>[12x]SVDTMALWLGLRAVLVVAGLAVLLQLIRGWLSSKSYVFNREEIARLAKEHSGLDYEVAFSKI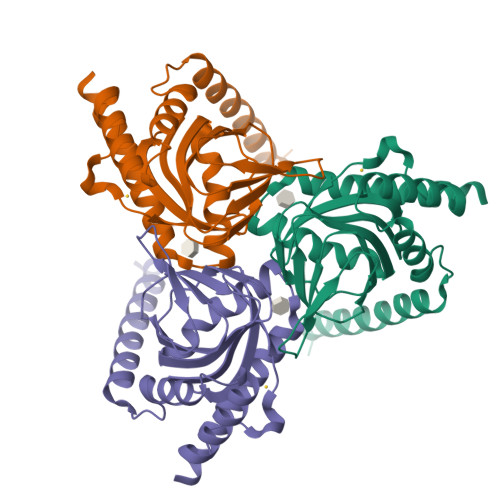IVELRKKHPGHILQDEDLQWVFVNAGGWMGSMCLLHASLTEYVLLFGTAVDTGGHSGRYWAEISDTILSGTFRQWKEGTTKSEIFYPGDTIVHEVGEATSVQWSSGTWMVEYGRGFIPSTLAFALADTIFSTQDFLTLFYTVKVYSKALLLEASTHLSQLGFF>[3x]MNREEMTLLGFEIVAYAGDARSKLLEALKAAENGDFA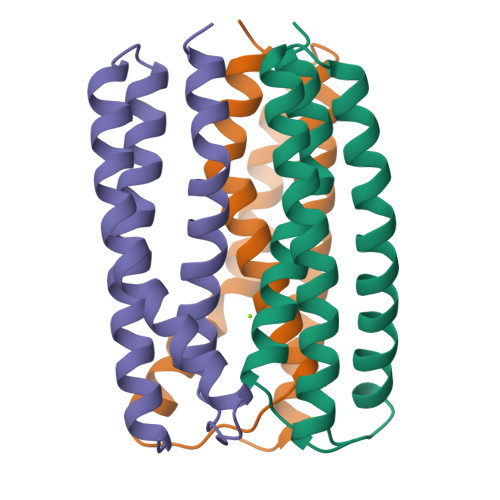KADSLVVEAGSCIAEAHSSQTGMLAREASGEELPYSVTMMHGQDHLMTTILLKDVIHHLIELYKRGAK> CDLNINDDPNYPMNDQVTADLIFPSISASIASAVGGEIYNYAGFFAQYYEQKPESNQYNTLCEYTFTESSQQMDYSYRILFAGALEDA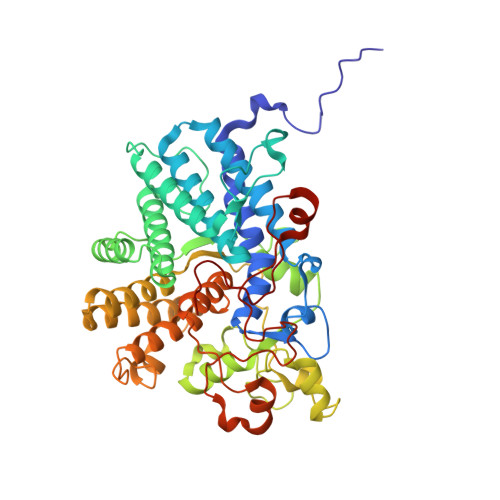KQVLEKTTNPADRFATTILRAYAFQIMVDNTSDSPYSEALQGNANATPKWDTGETVYKGILGEIDAAEAALDGSGMDVPDLIFNKNIAQWKGFANALRLRMYLRFIDANIDAASYTEKVKTLVQNNEFFTGDVKLDCFLDETDKRNPWYNTNAVGLTGNHCAAYPLVSYLSSTGDPRIAYGISKTDADGKYVGQLPGGKTHMQSILGTDNWKNKNVSAIDYSIGATKPVYFFTQAELQFLIAEVYARFHNDDANAKSAYEAGVTADFAVRGFAGQENTILEGACAWSAASTQADKLNLIYMQKWVSLFYMDHMEAWSEIRRTDCPKLSSYSAAQIQASESVYTPGELVAPWTNGLEAGGLMKRMTYPLSARQQNVNTPAGVPGSTPVWWDIK> EDKCSPSGAICSGAGP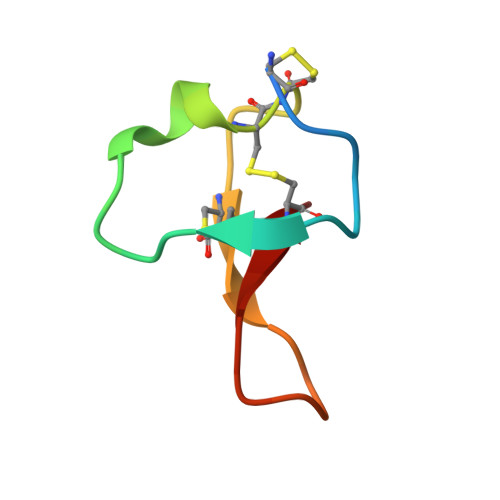PEQCCSGACVPHPILRIFVCQ>ATQGVFTLPANTRFGVTAFANSSGTQTVNVLVNNETAATFSGQSTNNAVIGTQVLNSGSSGKVQ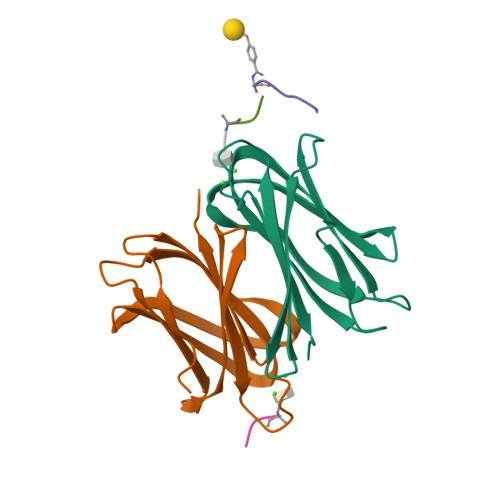VQVSVNGRPSDLVSAQVILTNELNFALVGSEDGTDNDYNDAVVVINWPLG[2x];> APAKFC;>APA[2x]>MAQLTQMTNEQLRELIEAVRAAAVGAAGSAAAAGGADASRGKGNFSACTHSFGGTRDHDVVEEFIGNIETYKDVEGISDENALKGISLLFYGMASTWWQGVRKEATTWKEAIALIREHFSPTKPAYQIYMEFFQNKQDDHDPIDTFVIQKRALLAQLPSGRHDEETELDLLFGLLNIKYRKHISRHSVHTFKDLLEQGRIIEHNNQEDEEQLATAKNTRGSKRTTRCTY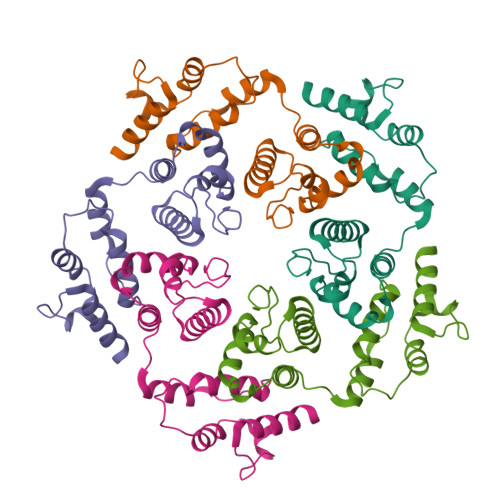CSFRGHTFDNCRKRQKDRQEEQHEE[5x]> MLPYMDQVLRAFYQSTHWSTQNSYEDITATSRTLLDFRIPSAIHLQISNKSTPNTFNSLDFSTRSRINGSLSYLYSDAQQLEKFMRNSTDIPLQDATETYRQLQPNLNFSVSSANTLSSDNTTVDNDKKLLHDSKFVKKSLYYGRMYYPSSDLEAMIIKRLSPQTQFMLKGVSS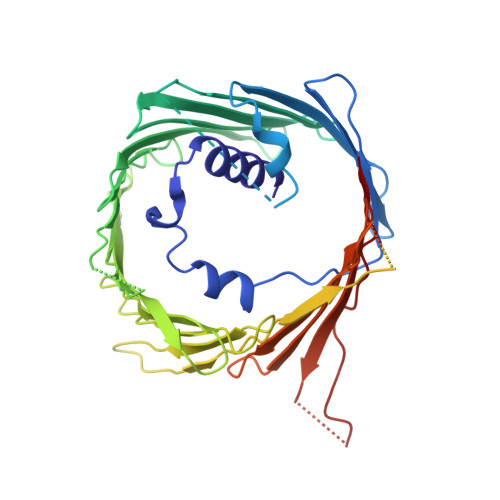FKESLNVLTCYFQRDSHRNLQEWIFSTSDLLCGYRVLHNFLTTPSKFNTSLYNNSSLSLGAEFWLGLVSLSPGCSTTLRYYTHSTNTGRPLTLTLSWNPLFGHISSTYSAKTGTNSTFCAKYDFNLYSIESNLSFGCEFWQKKHHLLETNKNNNDKLEPISDELVDINPNSRATKLLHENVPDLNSAVNDIPSTLDIPVHKQKLLNDLTYAFSSSLRKIDEERSTIEKFDNKINSSIFTSVWKLSTSLRDKTLKLLWEGKWRGFLISAGTELVFTRGFQESLSDDEKNDNAISISATDTENGNIPVFPAKFGIQFQYST>[2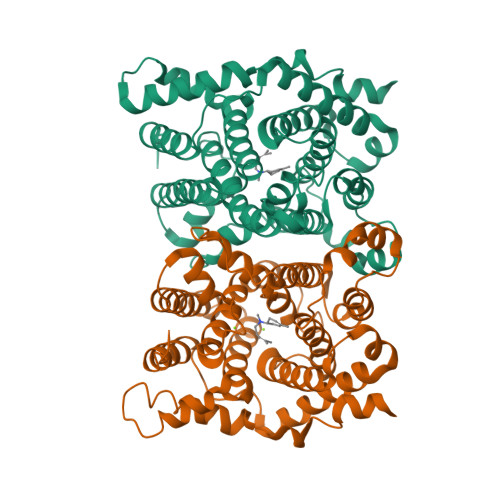x]MENFPTEYFLNTTVRLLEYIRYRDSNYTREERIENLHYAYNKAAHHFAQPRQQQLLKVDPKRLQASLQTIVGMVVYSWAKVSKECMADLSIHYTYTLVLEDSKDDPYPTMVNYFDDLQAGREQAHPWWALVNEHFPNVLRHFGPFCSLNLIRSTLDFFEGCWIEQYNFGGFPGSHDYPQFLRRMNGLGHCVGASLWPKEQFNERSLFLEITSAIAQMENWMVWVNDLMSFYKEFDDERDQISLVKNYVVSDEISLHEALEKLTQDTLHSSKQMVAVFSDKDPQVMDTIECFMHGYVTWHLCDRRYRLSEIYEKVKEEKTEDAQKFCKFYEQAANVGAVSPSEWAYPPVAQLANVRSKDVKEVQKPFLSSIELVE>[2x]MTRDQNGTWEMESNENFEGYMKALDIDFATRKIAVRLTQTKVIDQDGDNFKTKTTSTFRNYDVDFTVGVEFD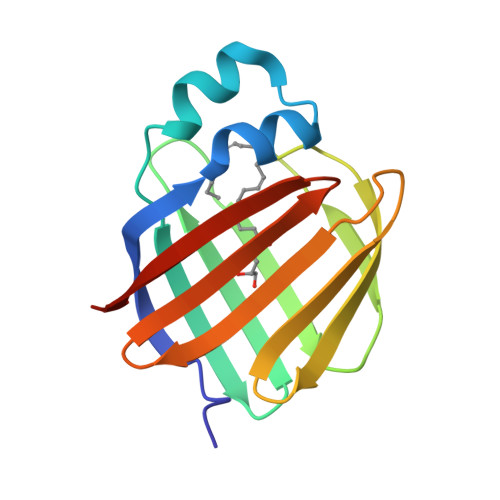EYTKSLDNRHVKALVTWEGDVLVCVQKGEKENRGWKQWIEGDKLYLELTCGDQVCRQVFKKKLVPR The findings presented in this manuscript highlight mechanistic and structural insights for D. melanogaster AgmNAT, an enzyme that catalyzes the formation of N-acetylagmatine from acetyl-CoA and agmatine. AgmNAT is a member of the GCN5-related N-acetyltransferase family (GNAT)2 and, in addition to the formation of N-acetylagmatine, this enzyme also catalyzes the production of N-acylpolyamines from the corresponding acyl-CoA and polyamine. As observed for arcaine, arginine methyl ester produced uncompetitive and competitive inhibition plots for acetyl-CoA and agmatine. These data demonstrate that AgmNAT catalyzes the formation of N-acetylagmatine through an ordered sequential mechanism: acetyl-CoA binding first followed by agmatine to generate the AgmNAT•acetyl-CoA•agmatine complex prior to catalysis. After the ternary complex formation, Glu-34 functions as the general base to deprotonate the positively charged amine moiety of agmatine, most likely involving a “proton wire” of ordered water molecules, followed by nucleophilic attack of the carbonyl of the acetyl-CoA thioester to generate a zwitterionic tetrahedral intermediate.

The AgmNAT (CG15766) crystal structure was determined at 2.3Å, with two monomers in the asymmetric unit of the P21 space group. The two monomers are nearly identical with an RMSD value of 0.262 Å when aligning 862 backbone atoms. Similar to the arylalkylamine N-acetyltransferase model, the new structure is primarily composed of six α-helices and seven anti-parallel α-strands. The active site is well defined in the 2Fo-Fc electron density map and is located near the crystal packing interface for both monomers. Moreover, a conserved glutamate, Glu-34, that serves as the catalytic base for other D. melanogaster N-acyltransferase enzymes, is located within an accessible pocket that can accommodate the acyl-CoA and amine substrate, similar to that observed for AANATA. Although only a number of water molecules (36 in total) were sufficiently ordered to be modeled in the current structure, the majority of them are in the active sites of the two monomers. The closest ordered water molecules to Glu-34 is ~ 3.7 Å from the Oε1, positioned slightly too far for a hydrogen bond; however, we anticipate that the conformational changes upon substrate binding could promote hydrogen bond interactions between ordered water molecules and the functional groups in AgmNAT and substrate. In addition, unlike Glu-33, which is exposed to the bulk solvent, Glu-34 is relatively sheltered and placed close to the hydrophobic core of the protein and next to residues such as Leu-36. In the current AgmNAT structure, Pro-35 is stacked on top of the imidazole ring of His-206 side chain.

>MAKPIADDIVVRQVDVGETEQLMTFLLAHYYPEEPLTAGTHPPEPEAADKEFLLSNVPFGTCFVALHEGRIVAAVVAGPKDSHEPEHMAEEARKYAGGKWGSILHLLSAVETATDVCRRFSVPSCLHVHALGVDPQLRGRNLGGRLMETVAQRGRDLGHQLVSVDCTSVYSARLVQRLGYQLINTLRYVDHLDASGQQVIRPPPPHESVQTFVLHL[2x]> GSHMEEVSEYCSHMIGSGHLQSLQRLIDSQMETSCQITFEFVDQEQLKDPVCYLKK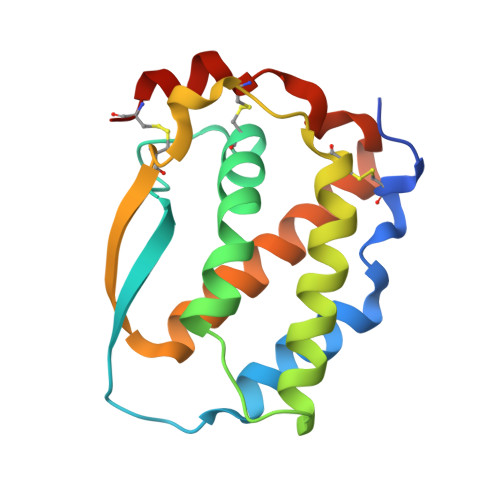AFLLVQDIMEDTMRFRDNTPNAIAIVQLQELSLRLKSCFTKDYEEHDKACVRTFYETPLQLLEKVKNVFNETKNLLDKDWNIFSKNCNNSFAECSSQ> MELAEKDKGRDFTLRNARMDDIDQIIKINRLTLPENYPYYFFVEHLKEYGLAFFVAIVDNSVVGYIMPRIEWGFSNIKQLPSLVRKGHVVSIAVLEEYRRKGIATTLLEASMKSMKNDYNAEEIYLEVRVSNYPAIALYEKLNFKKVKVLKGYYADGEDAYLMARPLHHHHHH

Nα-acetyltransferase (Nat) performs this modification and transfers an acetyl group from acetyl-coenzyme A (acetyl-CoA) to an α-amino group from the first residue of the protein substrate. A BLAST search identified Ard1 from Crenarchaeal Sulfolobus solfataricus (SsArd1) as a homolog of the Ard1 subunit of yeast NatA and Naa10p subunit of human NatA. However, no Sulfolobus homolog of the auxiliary subunit of NatA was found, so SsArd1 alone may be responsible for the protein acetylation. SsArd1 has a mixed α/β-fold with 7 β-sheet surrounded by 4 α-helices and contains 4 conserved motifs, a feature unique to the GCN5-related N-acetyltransferase (GNAT) family.

The crystal structure of the SsArd1-CoA binary complex was determined at 2.13 Å resolution and the SsArd1–CoA/peptide ternary complex at 1.84 Å. CoA-bound and CoA/peptide-bound SsArd1 structures were almost identical and could be superimposed, with root mean square deviation (RMSD) 0.12 Å for all Cα atoms. The CoA is bound to SsArd1 in a bent conformation in the pyrophosphate region, for pantetheine fitting to the narrow central cleft and the acetyl group reaching the midpoint of the tunnel. In the complex structure, the adenosine 3′-phosphate group of CoA is placed on the outside of the tunnel entrance and exposed to the protein surface. Adenosine 3′-phosphate, pyrophosphate and pantothenic acid of CoA contact SsArd1 via many van der Waals interactions and hydrogen bonds. The main-chains of Ile92, Val94, Arg100, Gly102, Ala104 and Thr105 contribute to hydrogen bonding with CoA. The side-chains of Arg100, Thr105 and Asn132 contact with the 3′-phosphate of adenosyl moiety, pyrophosphate and pantothenic acid, respectively, by hydrogen bonds. The crystal structure of SsArd1 in complex with CoA revealed that Arg100 was the only residue contributing two hydrogen bonds to the 3′-phosphate of adenosyl moiety. The side-chain of Arg100 served as a position of adenosine moiety of CoA located at the cave formed by the α4 and β4-α3 loop. In contrast, the positive-charged guanidino group of the Arg100 residue of SsArd1 occupied the space and formed a cation-pi interaction with the adenosine group of CoA, which may force the acetyl group less deep into the catalytic pocket for larger protein N-terminal residues.> EGDIHMKKGHHHHHHENLYFQGGSGKLSEQLKHCNGILKELLSKKHAAYAWPFYKPVDASALGLHDYHDIIKHPMDLSTVKRKMENRDYRDAQEFAADVRLMFSNCYKYNPPDHDVVAMARKLQDVFEFRYA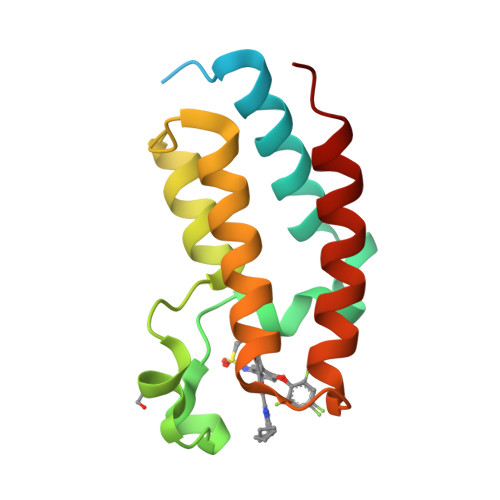KMPD> FPTIPLSRLFDNAMLRAHRLHQLAFDTYQEFEEAYIPKEQKYSFLQNPQTSLCFSESIPTPSNREETQQKSNLELLRISLLLIQSWLEPVQFLRSVFANSLVYGASDSNVYDLLKDLEEGIQTLMGRLEDGSPRTGQIFKQTYSKFDTNSHNDDALLKNYGLLYCFRKDMDKVETFLRIVQCRSVEGSCG;>[2x]EPKFTKCR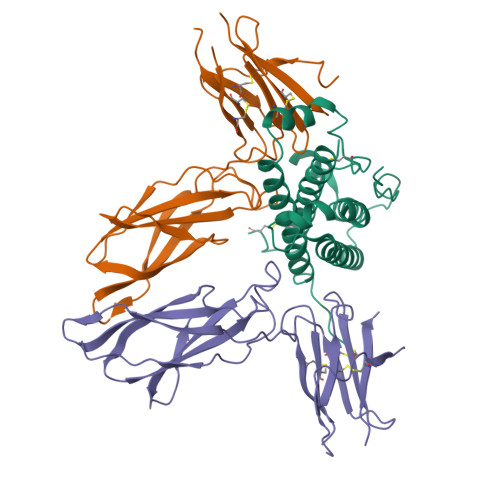SPERETFSCHWTDEVHHGTKNLGPIQLFYTRRNTQEWTQEWKECPDYVSAGENSCYFNSSFTSIWIPYCIKLTSNGGTVDEKCFSVDEIVQPDPPIALNWTLLNVSLTGIHADIQVRWEAPRNADIQKGWMVLEYELQYKEVNETKWKMMDPILTTSVPVYSLKVDKEYEVRVRSKQRNSGNYGEFSEVLYVTLPQM> TTLLNPYFGEFGGMYVPQILMPALNQ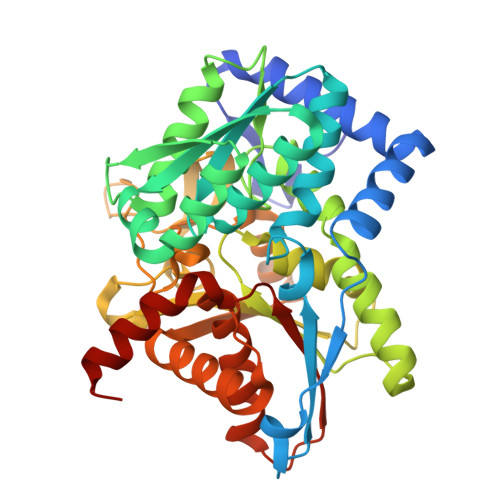LEEAFVSAQKDPEFQAQFADLLKNYAGRPTALTKCQNITAGTRTTLYLKREDLLHGGAHKTNQVLGQALLAKRMGKSEIIAETGAGAHGVASALASALLGLKCRIYMGAKDVERQSPNVFRMRLMGAEVIPVHSGSATLKDACNEALRDWSGSYETAHYMLGTAAGPHPYPTIVREFQRMIGEETKAQILDKEGRLPDAVIACVGGGSNAIGMFADFINDTSVGLIGVEPGGHGIETGEHGAPLKHGRVGIYFGMKAPMMQTADGQIEESYSISAGLDFPSVGPQHAYLNSIGRADYVSITDDEALEAFKTLCRHEGIIPALESSHALAHALKMMREQPEKEQLLVVNLSGRGDKDIFTVHDILKARGE> MSRKRSTKPKPAAKIALKKYNDQFLEALKLYEGKQYKKSLKLLDAILKKDGSHVDSL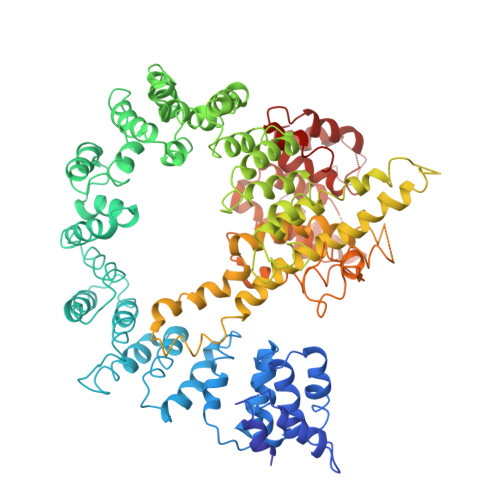ALKGLDLYSVGEKDDAASYVANAIRKIEGASASPICCHVLGIYMRNTKEYKESIKWFTAALNNGSTNKQIYRDLATLQSQIGDFKNALVSRKKYWEAFLGYRANWTSLAVAQDVNGERQQAINTLSQFEKLAEGKISDSEKYEHSECLMYKNDIMYKAASDNQDKLQNVLKHLNDIEPCVFDKFGLLERKATIYMKLGQLKDASIVYRTLIKRNPDNFKYYKLLEVSLGIQGDNKLKKALYGKLEQFYPRCEPPKFIPLTFLQDKEELSKKLREYVLPQLERGVPATFSNVKPLYQRRKSKVSPLLEKIVLDYLSGLDPTQDPIPFIWTNYYLSQHFLFLKDFPKAQEYIDAALDHTPTLVEFYILKARILKHLGLMDTAAGILEEGRQLDLQDRFINCKTVKYFLRANNIDKAVEVASLFTKNDDSVNGIKDLHLVEASWFIVEQAEAYYRLYLDRKKKLDDLASLKKEVESDKSEQIANDIKENQWLVRKYKGLALKRFNAIPKFYKQFEDDQLDFHSYCMRKGTPRAYLEMLEWGKALYTKPMYVRAMKEASKLYFQMHDDRLKRKSDSLDENSDEIQNNGQNSSSQKKKAKKEAAAMNKRKETEAKSVAAYPSDQDNDVFGEKLIETSTPMEDFATEFYNNYSMQVREDERDYILDFEFNYRIGKLALCFASLNKFAKRFGTTSGLFGSMAIVLLHATRNDTPFDPILKKVVTKSLEKEYSENFPLNEISNNSFDWLNFYQEKFGKNDINGLLFLYRYRDDVPIGSSNLKEMIISSLSPLEPHSQNEILQYYL>HHHHHHMSKRETFNETFLKAARGEKADHTPVWYMRQAGRSQPEYRKLKEKYGLFEITHQPELCAYVTRLPVEQYGVDAAILYKDIMTPLPSIGVDVEIKNGIGPVIDQPIRSLADIEKLGQIDPEQDVPYVLETIKLLVNEQLNVPLIGFSGAPFTLASYMTEGGPSKNYNKTKAFMYSMPDAWNLLMSKLADMIIVYVKAQIKAGAKAIQIFDSWVGALNQADYRTYIKPVMNRIFSELAKENVPLIMFGVGASHLAGDWHDLPLDVVGLDWRLGIDEARSKGITKTVQGNLDPSILLAPWEVIEQKTKEILDQGMESDGFIFNLGHGVFPDVSPEVLKKLTAFVHEYSQNKKMGQ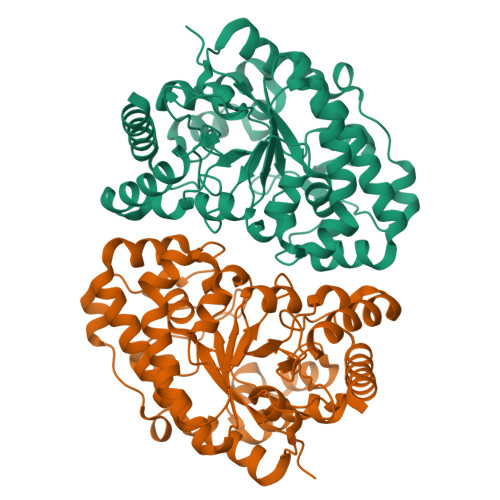YS[4x]>[2x]STAGKVIKCKAAVLWELKKPFSIEEVEVAPPKAHEVRIKMVAAGICRSDEHVVSGNLVTPLPVILGHEAAGIVESVGEGVTTVKPGDKVIPLFTPQCGKCRICKNPESNYCLKNDLGNPRGTLQDGTRRFTCSGKPIHHFVGVSTFSQYTVVDENAVAK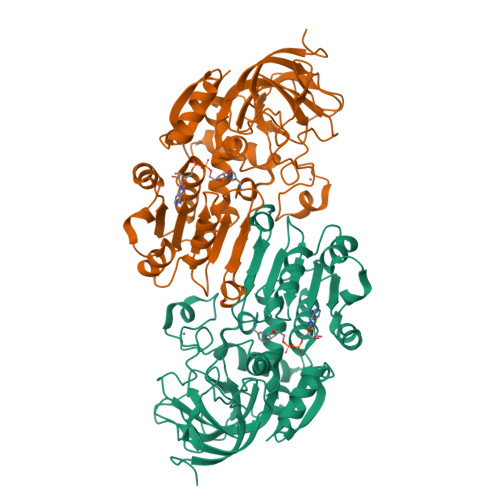IDAASPLEKVCLIGCGFSTGYGSAVKVAKVTPGSTCAVFGLGGVGLSVVMGCKAAGAARIIAVDINKDKFAKAKELGATECINPQDYKKPIQEVLKEMTDGGVDFSFEVIGQLDTMMASLLCCHEACGTSVIVGVPPDSQNLSINPMLLLTGRTWKGAIFGGFKSKESVPKLVADFMAKKFSLDALITNVLPFEKINEGFDLLRSGKSIRTVLTF> GSNVPTGLTGNFREDTLALISSLREAIALPENDPNKKAAQAEARKKLNDFFALYRRDDSLRSLSSFMTMQTALNSLAGHYSSYPNRPLPEKLKARLEQE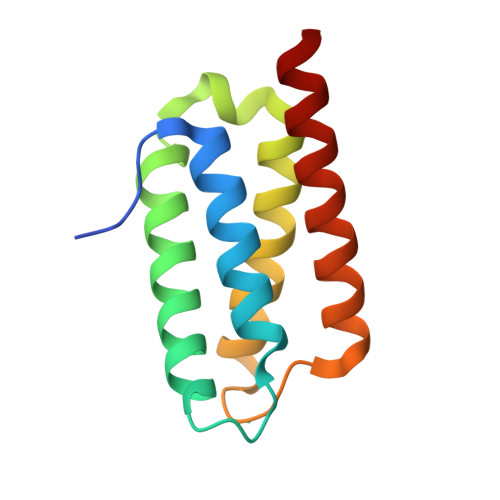FKQVELALDREAKS3-[(cyclohexanecarbonyl)amino]-N-(2,3-dihydro-1H-inden-2-yl)pyrazine-2-carboxamide | C21 H24 N4 O2 | 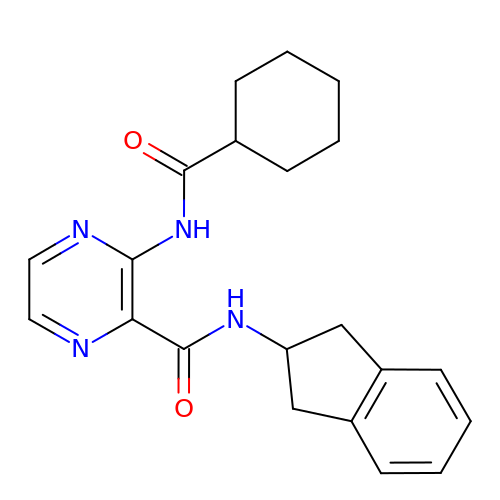OOCYBEPYZJOAIY-UHFFFAOYSA-N> MAVTNEEIKTASKIVRRVSNVEAFDKSGSVFKGYQIWTDISPTIENDPNIMFVKCVVQQGSKKEKLTVVQIDPPGTGTPYDIDPTHAWNCNSQVDPMSFGDIGLLNHTNIPCVLDFLKHRYLKNQIYTTAVPLIVAINPYKDLGNTTNEWIRRYRDTADHTKLPPHVFTCAREALSNLHGVNKSQTIIVSGESGAGKTEATKQIMRYFASSKSGNMDLRIQTAIMAANPVLEAFGNAKTIRNNNSSRFGRFMQLVISHEGGIRYGSVVAFLLEKSRIITQDDNERSYHIFYQFLKGANSTMKSKFGLKGVTEYKLLNPNSTEVSGVDDVKDFEEVIESLKNMELSESDIEVIFSIVAGILTLGNVRLIEKQEAGLSDAAAIMDEDMGVFNKACELMYLDPELIKREILIKVTVAGGTKIEGRWNKNDAEVLKSSLCKAMYEKLFLWIIRHLNSRIEPEGGFKTFMGMLDIFGFEVFKNNSLEQLFINITNEMLQKNFVDIVFERESKLYKDEGISTAELKYTSNKEVINVLCEKGKSVLSYLEDQCLAPGGTDEKFVSSCATNLKENNKFTPA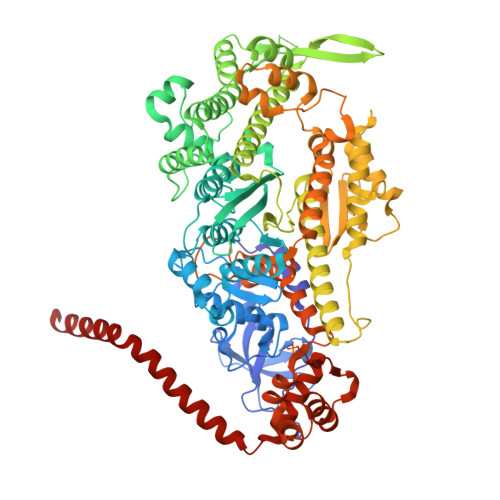KVASNKNFIIQHTIGPIQYCAESFLLKNKDVLRGDLVEVIKDSPNPIVQQLFEGQVIEKGKIAKGSLIGSQFLNQLTSLMNLINSTEPHFIRCIKPNENKKPLEWCEPKILIQLHALSILEALVLRQLGYSYRRTFEEFLYQYKFVDIAAAEDSSVENQNKCVNILKLSGLSESMYKIGKSMVFLKQEGAKILTKIQREKLVEWENCVSVIEAAILKHKYKQKVNKNIPSLLRVQAHIRKKMVAQ1,3-dimethyl-8-{[2-(pyrrolidin-1-yl)ethyl]sulfanyl}-6-sulfanylidene-1,3,6,9-tetrahydro-2H-purin-2-one 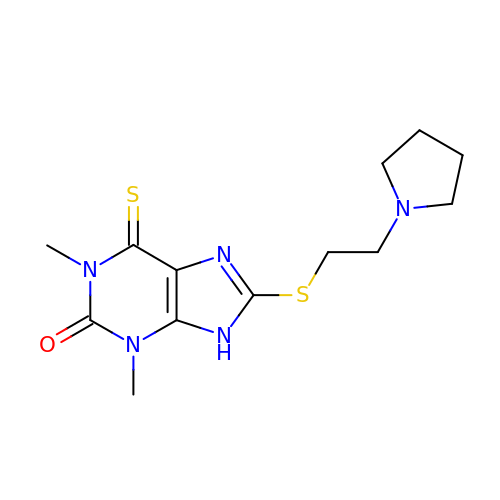| C13 H19 N5 O S2 | KLAIFKHPSDRWRR-UHFFFAOYSA-N> RLSR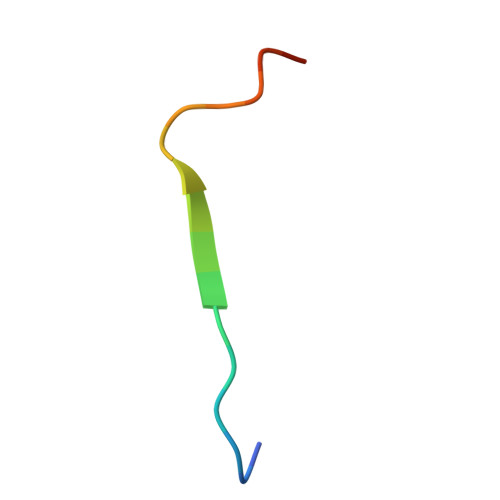KTHMYPVRNYSPTE>[4x]GSESSRSAMMYIQELRSGLRDMHLLSCLESLRVSLNNNPVSWVQTFGAEGLASLLDILKRLHDEKEETSGNYDSRNQHEIIRCLKAFMNNKFGIKTMLETEEGILLLVRAMDPAVPNMMIDAAKLLSALCILPQPEDMNERVLEAMTERAEMDEVERFQPLLDGLKSGTSIALKVGCLQLINALITPAEELDFRVHIRSELMRLGLHQVLQELREIENEDMKVQLCVFDEQGDEDFFDLKGRLDDIRMEMDDFGEVFQIILNTVKDSKAEPHFLSILQHLLLVRNDYEARPQYYKLIEECVSQIVLHKNGTDPDFKCRHLQIDIERLVDQ;>GSFGFGVPAAPVLPFGLTPKKVYKPEVQLRRPNWSKFVAEDLSQDCFWTKVKEDRFENNELFAKLTLAFSAQTKTSKAKKDQEGGEEKKSVQKKKVKELKVLDSKTAQNLSIFLGSFRMPYQEIKNVILEVNEAVLTESMIQNLIKQMPEPEQLKMLSELKEEYDDLAESEQFGVVMGTVPRLRPRLNAILFKLQFSEQVENIKPEIVSVTAACEELRKSENFSSLLELTLLVGNYMNAGSRNAGAFGFNISFLCKLRDTKSADQKMTLLHFLAELCENDHPEVLKFPDELAHVEKASRVSAENLQKSLDQMKKQIADVERDVQNFPAATDEKDKFVEKMTSFVKDAQEQYNKLRMMHSNMETLYKELGDYFVFDPKKLSVEEFFMDLHNFRNMFLQAVKENQKRRETEEKMRRAKLAKEKAEKERLEKQQKREQLIDMNAEGDETGVMDSLLEALQSGAAFRRKRG[4x]

Formin proteins direct the nucleation and assembly of linear actin filaments in a variety of cellular processes using their conserved formin homology 2 (FH2) domain. Diaphanous-related formins (DRFs) are effectors of Rho-family GTPases, and in the absence of Rho activation they are maintained in an inactive state by intramolecular interactions between their regulatory N-terminal region and a C-terminal segment referred to as the DAD domain. Biochemically, the FH2 domain potently nucleates new, unbranched actin filaments and remains attached to the growing barbed end of the filament as additional actin subunits are incorporated. The mammalian DRF Dia1 is important for stress fiber assembly and cell migration.

We crystallized and determined the structure of an “N+C” complex containing the N-terminal DID and DD domains (DID-DD) bound to the C-terminal FH2-DAD construct. We obtained crystals of the DID-DD protein in complex with FH2-DAD in space group P21 and determined the structure by molecular replacement using available structures of the mDia1 N-terminus and truncated FH2 domain as search models. The structure was refined to a crystallographic R-value of 23.7% (Rfree = 29.6%) using data extending to 3.2 Å resolution. The crystals contain two dimeric N+C complexes in the asymmetric unit, where each of these dimers is in turn composed of a dimeric N-terminal fragment bound to a dimeric C-terminal fragment via interactions of their respective DID and DAD domains. As we discuss more fully below, we cannot unambiguously determine the pairing of C-terminal FH2 domain fragments into dimers. The tetramer has approximate 222 point symmetry, and is composed of two symmetrically interlocked N+C dimers, as illustrated in Figure 1B. The tetramer effectively consists of four layers; two FH2 dimers form the two central layers, while the N-terminal dimers pack on either side to form the two outer layers. This interlocked structure is held together primarily, if not entirely, by the interactions of the DID domains of each N-terminal dimer with the DAD domains emanating from the more distal FH2 dimer. An ∼85 Å long α-helix (αT) extends from the post of the FH2 domain, and the autoregulatory DAD domain segment is connected to the end of helix αT by a 10-residue loop segment. In the present structure, all four flexible linkers are disordered, complicating assignment of the connectivity of the FH2 domain dimers. The DAD is composed of a core helical region with the sequence motif “MDXLLXL” and an adjacent basic segment with the sequence “RRKR” in mDia1. The interactions of the DAD domain with the DID are essentially the same as previously described for structures containing the isolated DAD segment, but additional interactions are observed for the basic C-terminal portion of the DAD. In the tetramer, the FH2 domains pack back-to-back, with their actin binding surfaces facing outward (up on one FH2 domain and down on the other in the orientation presented here).>[2x]GSSHHHHHHMSSFQLPKLSYDYDELEPYIDSNTLSIHHGKHHATYVNNLNAALENYSELHNKSLEELLCNLETLPKEIVTAVRNNGGGHYCHSLFWEVMSPRGGGEPNGDVAKVIDYYF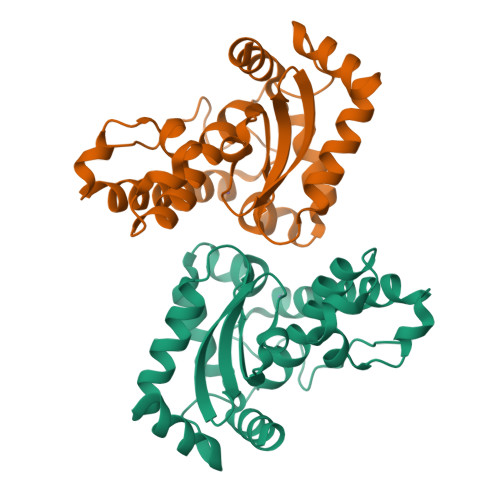NTFDNLKDQLSKAAISRFGSGYGWLVLDGEELSVMSTPNQDTPLQEGKIPLLVIDVWEHAYYLKYQNRRPEFVTNWWHTVNWDRVNEKYLQAIQSQKH> CACGCG;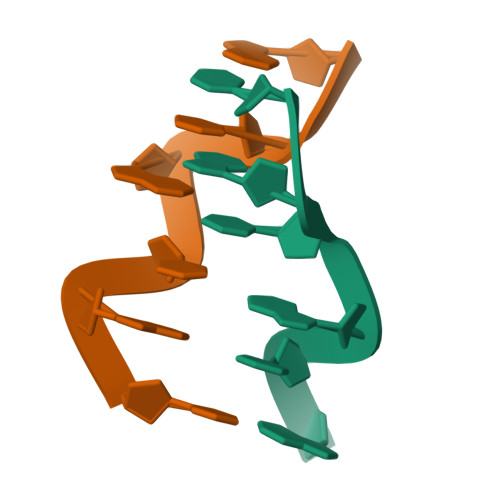> CGCGTG;>[2x]TG>[2x]MMIVQRVVLNSRPGKNGNPVAENFRMEEVYLPDNINEGQVQVRTLYLSVDPYMRCRMNEDTGTDYITPWQLSQVVDGGGIGIIEESKHTNLTKGDFVTSFYWPWQTKVILDGNSLEKVDPQLVDGHLSYFLG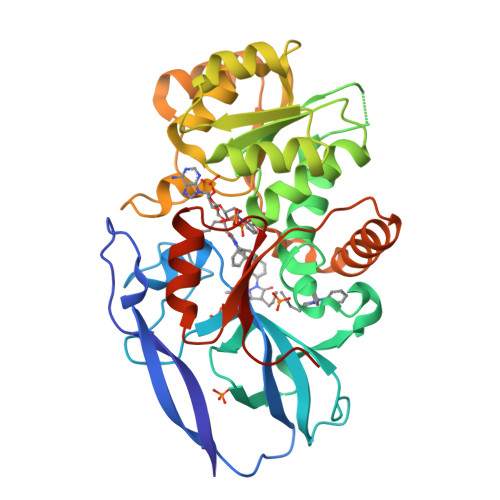AIGMPGLTSLIGIQEKGHITAGSNKTMVVSGAAGACGSVAGQIGHFLGCSRVVGICGTHEKCILLTSELGFDAAINYKKDNVAEQLRESCPAGVDVYFDNVGGNISDTVISQMNENSHIILCGQISQYNKDVPYPPPLSPAIEAIQKERNITRERFLVLNYKDKFEPGILQLSQWFKEGKLKIKETVINGLENMGAAFQSMMTGGNIGKQIVCISEEIAENLYFQ[5-hydroxy-4-(methoxymethyl)-6-methylpyridin-3-yl]methyl dihydrogen phosphate | C9 H14 N O6 P | 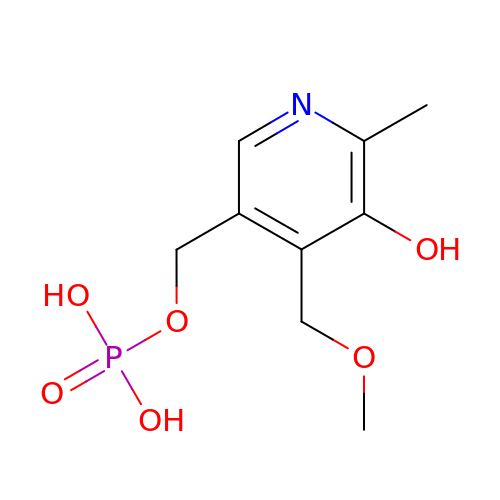RFYDYCIMPLKICN-UHFFFAOYSA-N> RKREASLITLNYIKNRFYPSK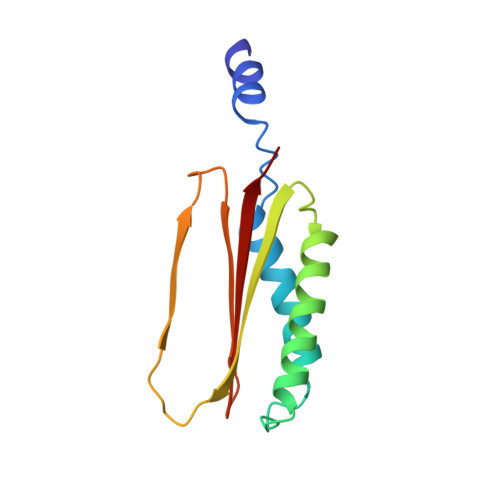IQKIIKELFEDRLKGVEYDPNNANQLSERLVLELREKIKRGKVPRYKIGVQVVFGEIKGQGLRIASKCLWDVQNDNYASYTYTSEKVYCTGIVFGCYFE> XEYEYE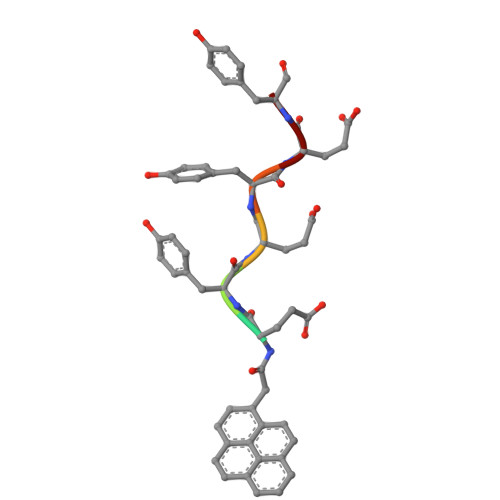Y>[8x]GSEELLDLFNRQVTQEFTASQVYLSASIWFDQNDWEGMAAYMLAESAEEREHGLGFVDFANKRNIPIELQAVPAPVSCA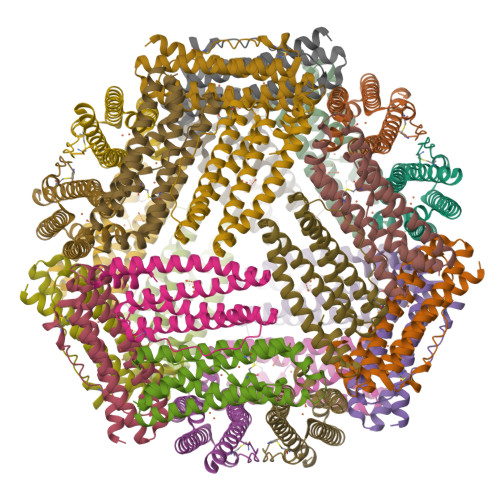EWSSPEDVWQSILELEQANTRSLLNLAEAASTCHDFAVMAFLNPFHLQQVNEEDKIGSILAKVTDENRTPGLLRSLDVVSFLGPCLFRS>ASMTGGQQMGAPITAYAQQTRGLLGCIITSLTGRDKNQVEGEVQIVSTATQTFLATCINGVCWTVYHGAGTRTIASPKGPVIQMYTNVDQDLVGWPAPQGSRSLTPCTCGSSDLYLVTRHADVIPVRRRGDSRGSLLSPRPISYLKGSAGGPLLCPAGHAVGLFRAAVCTRGVAKAVDFIPVENLETTMRGSHHHHHH[2x];>[2x]K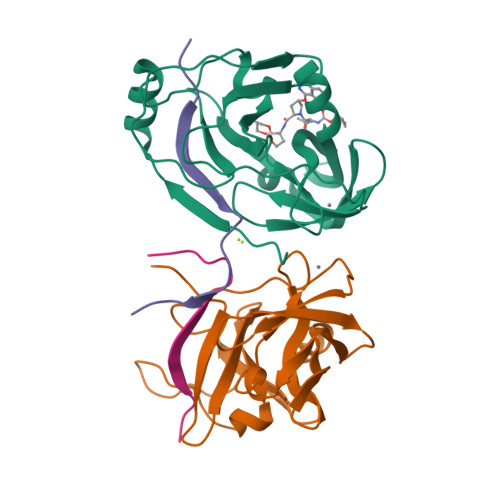KGSVVIVGRIVLSGKPAIIPKK>MSITLSDSAAARVNTFLANRGKGFGLRLGVRTSGCSGMAYVLEFVDEPTPEDIVFEDKGVKVVVDGKSLQFLDGT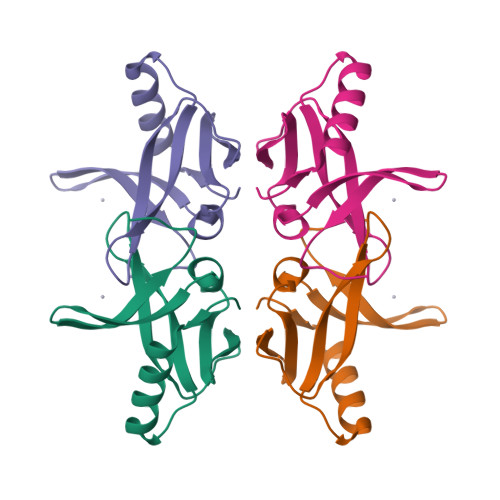QLDFVKEGLNEGFKFTNPNVKDECGCGESFKLAAALDHHHHHH[2x]> T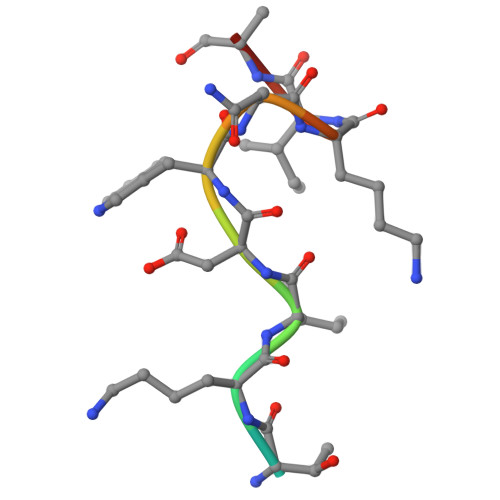RTKIDWNKILS>[2x]TPEGLSSEQQRAFLAVTQTPHPAHLITGPAGTGKTTLLYALQKFYKG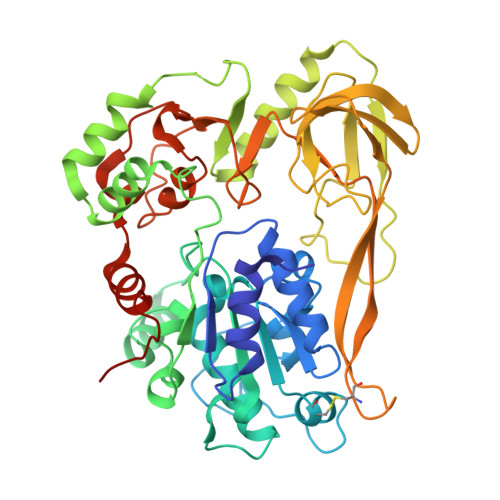RAVTLAPTGTAALQARGQTVHSFFRFPARLLRYRHPEDIRPPGPHSPLRKAIECMEVLILDEVGMVRVDLLEAMDWALRKTRKRLEEPFGGVKVLLLGDTRQLEPVVPGGEEALYIARTWGGPFFFQAHVWEEVALRVHRLWESQRQREDPLFAELLKRLRQGDPQALETLNRAAVRPDGGEEPGTLILTPRRKEADALNLKRLEALPGKPLEYQAQVKGEFAETDFPTEAALTLKKGAQVILLRNDPLGEYFNGDLGWVEDLEAEALAVRLKRNGRRVVIRPFVWEKIVYTYDSERECIKPQVVGTFRQVPVRLAWALTVHKAQGLTLDKVHLELGRGLFAHGQLYVALTRVRRLQDLSLSRPIAPTELLWRPEVEVFETRIQEGIWQKSHGWPSLVD>[4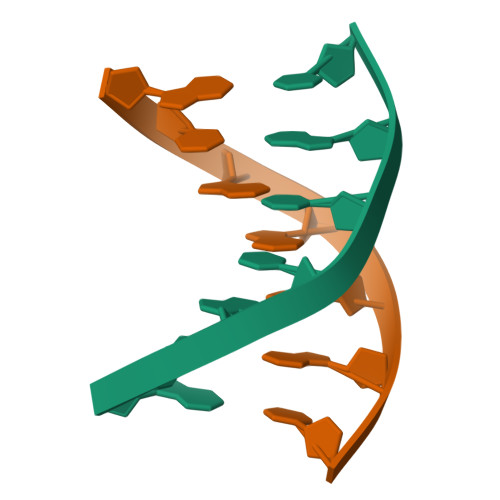x]ACGCCGT;>ACGGCGT[4x]>[2x]SPEGYQLEQVLIMSRANLRAPLANNGSVLEQSTPKQWPEWEVPGGQLTTKGGVLEVYMGHYMREWLAQQGMVKTGECPAADSVYAYANSLQRTVATAQFFITGAFPGCDVPVHHQEKMGTMDPTFNPVITDNSPEFREKA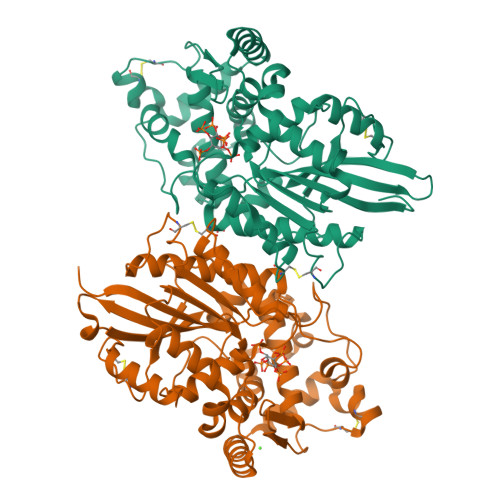LKAMETERQKMQLTESYKLLEQMTNYADSPSCKEKKVCSLADAKDTFSADYEKEPGVSGPLKVGNSLVDAFTLQYYEGFPADQVAWGEIKTDQQWRVLSKLKNGYQDSLFTSTEVAQNVAKPLVKYIDKTLVTEQAKAPKITLLVGHDSNIASLLTALDFKPYQLHDQQERTPIGGKIVFQRWHDKNANQELMKIEYVYQSSEQLRNASVLSLQSPAQRVTLELKGCPVDANGFCPVDKFNAVMNNAAKRSGHHHHHH>KKYRFIVYTGVPVTRIMAQSTDDAISLYDMPSQRFRYIEDENMNWTNLDSRWYSQNSLKAIPMIIVPVPQGEWTVEISMEGYQPTSSTTDPNKDKQDGLIAYNDDLSEGWNVGIYNNVEITNNKADNTLKYGHPDMELNGCHFNQGQCLERDGDLTCHIKTTGDNASFFVVGPAVQKQSKYNYA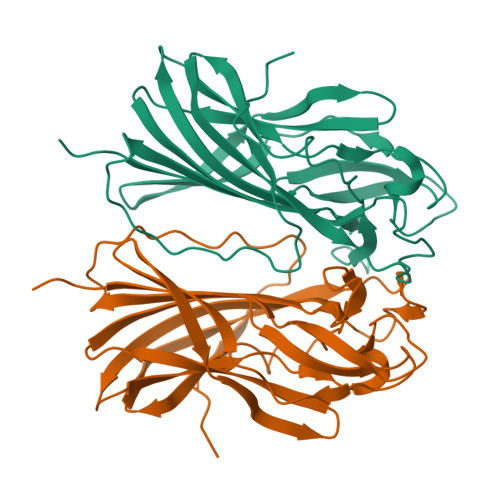VSYGAWTDRMMEIGMIAIALDEQGSSGSVKTERPKRVGHSMAVSTWETIKLPEK[2x]>[2x]MSGEQKSYLENQLEAVAEKTDAGYTFTFQREKIKLLDGLEANVIKDINPFFHKEIDVTDDEVIITIQPPSSYKAFRFMKAKDKKSKWQFAYQLVQ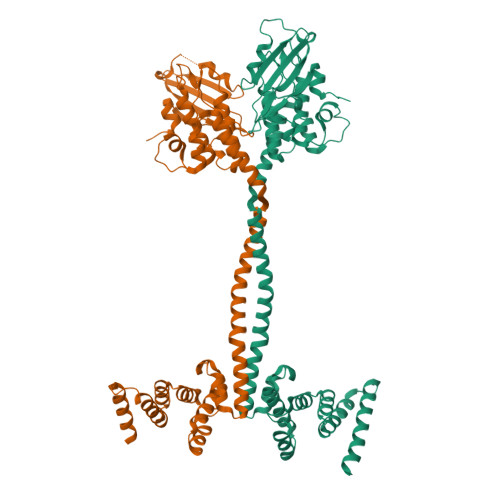AVQQHNLSRLNLIVAPENIVFDKGLTPYFLHYGVKESIPPYERDEERVWQELKAAAALAVDGAFAFEDYLKFNETLTFSAEAKAILDAESYDDLLELIQTHIDELEAKAKTYIHIPRKKWNIQRYIGLGLIVLLVPALIYSMYALFFAQPKHQAIVDSNRAFLNKQYSEVISTLSKYDAESLPESVQYQLATSYVEVENLGSAKTKNIENNLVTLQSDPQHFLYWIDYGRGEYKEAISIGRKLEYNDYIYFALAKYKQQLLSEDTNDEDIQKELDSVNSELEKAQKERQENKQSNSETSLVDTSEEQTQTDEEKQAEEWSHPQFEKAA9-AMINOPHENANTHRENE | C14 H11 N | 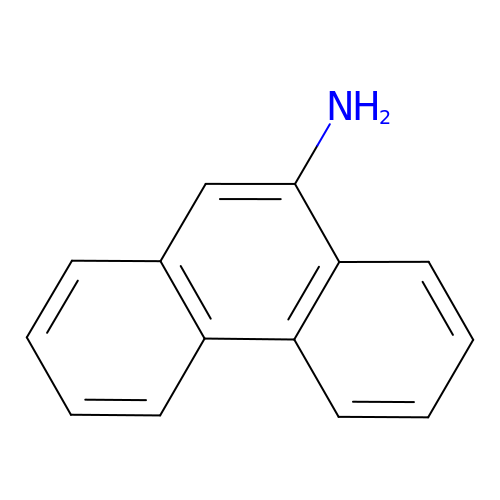KIHQWOBUUIPWAN-UHFFFAOYSA-N> CACGCG;>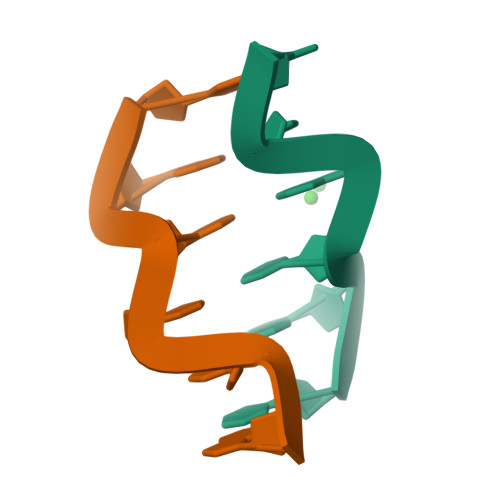 CGCGTG>CGVGFIANLRGKPDHTLVEQALKALGCMEHRGGCSADNDSGDGAGVMTAIPRELLAQWFNTRNLPMPDGDRLGVGMVFLPQEPSAREVARAYVEEVVRLEKLTVLGWREVPVNSDVLGIQAKNNQPHIEQILVTCPEGCAGDELDRRLYIARSIIGKKLAEDFYVCSFSCRTIVYKGMVRSIILGEFYLDLKNPGYTSNFAVYHRRFSTNTMPKWPLAQPMRLLGHNGE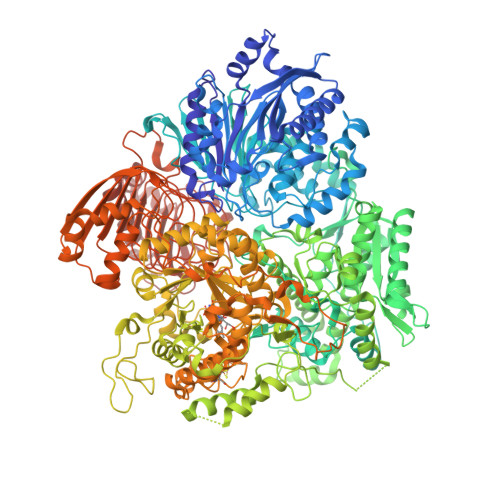INTLLGNINWMAAREKELEVSGWTKAELEALTPIVNQANSDSYNLDSALELLVRTGRSPLEAAMILVPEAYKNQPALKDYPEISDFHDYYSGLQEPWDGPALLVFSDGKIVGAGLDRNGLRPARYCITKDDYIVLGSEAGVVDLPEVDIVEKGRLAPGQMIAVDLAEQKILKNYQIKQQAAQKYPYGEWIKIQRQTVASDSFAEKTLFNDAQTVLQQQAAFGYTAEDVEMVVVPMASQGKEPTFCMGDDTPLAVLSHKPRLLYDYFKQRFAQVTNPPIDPLRENLVMSLAMFLGKRGNLLEPKAESARTIKLRSPLVNEVELQAIKTGQLQVAEVSTLYDLDGVNSLEDALTNLVKTAIATVQAGAEILVLTDRPNGAILTENQSFIPPLLAVGAVHHHLIRAGLRLKASLIVDTAQCWSTHHFACLVGYGASAICPYLALESVRQWWLDEKTQKLMENGRLDRIDLPTALKNYRQSVEAGLFKILSKMGISLLASYHGAQIFEAIGLGAELVEYAFAGTTSRVGGLTIADVAGEVMVFHGMAFPEMAKKLENFGFVNYRPGGEYHMNSPEMSKSLHKAVAAYKVGGNGNNGEAYDHYELYRQYLKDRPVTALRDLLDFNADQPAISLEEVESVESIVKRFCTGGMSLGALSREAHETLAIAMNRLGAKSNSGEGGEDVVRYLTLDDVDSEGNSPTLPHLHGLQNGDTANSAIKQIASGRFGVTPEYLMSGKQLEIKMAQGAKPGEGGQLPGKKVSEYIAMLRRSKPGVTLISPPPHHDIYSIEDLAQLIYDLHQINPEAQVSVKLVAEIGIGTIAAGVAKANADIIQISGHDGGTGASPLSSIKHAGSPWELGVTEVHRVLMENQLRDRVLLRADGGLKTGWDVVMAALMGAEEYGFGSIAMIAEGCIMARVCHTNNCPVGVATQQERLRQRFKGVPGQVVNFFYFIAEEVRSLLAHLGYRSLDDIIGRTDLLKVRSDVQLSKTQNLTLDCLLNLPDTKQNRQWLNHEPVHSNGPVLDDDILADPDIQEAINHQTTATKTYRLVNTDRTVGTRLSGAIAKKYGNNGFEGNITLNFQGAAGQSFGAFNLDGMTLHLQGEANDYVGKGMNGGEIVIVPHPQASFAPEDNVIIGNTCLYGATGGNLYANGRAGERFAVRNSVGKAVIEGAGDHCCEYMTGGVIVVLGPVGRNVGAGMTGGLAYFLDEVGDLPEKINPEIITLQRITASKGEEQLKSLITAHVEHTGSPKGKAILANWSDYLGKFWQAVPPSEKDSPEANNDVSLTGEKTLTSV[2x]>[2x]METIQELILSEENKTNIAVLNLGTNDRRNAVLILETALHLVEKYLGKII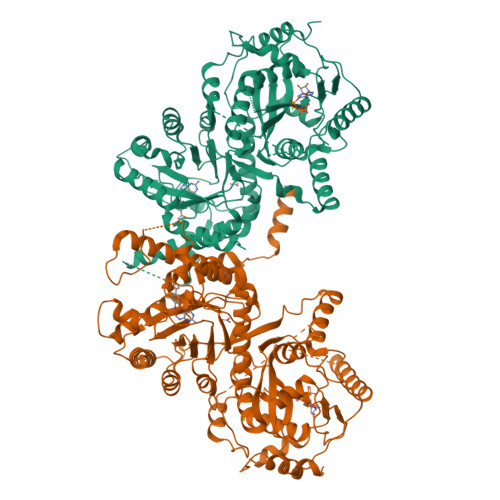NTSYLYETVPEYIVLDKKESCEKINKDCRIYDVNYINELMQNLEESKYEENKELIDKCEEYETFLKNGKVDNSILKEVNVENYLLECNNIIVKNDEIMKNNLSKYKDKYYTSYFYNLTVVVKTFVNDPLSMLVVIKYIEELMKRENVKEKEKFENRIIDIDILFFNDFTIFMKNIKLEKNMIYKILSKYIHLERDIKNGNDNMSKVNMDKDINLNNNNNIKKKNNNDIDCDCVDQKMNNHVNNKNYINSFRDPQEIINNMVDNIEFLSIPHVYTTHRYSILLCLNDMIPEYKHNVLNNTIRCLYNKYVSRMKEQYNINIKENNKRIYVLKDRISYLKEKTNIVGILNVNYDSFSDGGIFVEPKRAVQRMFEMINEGASVIDIGGESSGPFVIPNPKISERDLVVPVLQLFQKEWNDIKNKIVKCDAKPIISIDTINYNVFKECVDNDLVDILNDISACTNNPEIIKLLKKKNKFYSVVLMHKRGNPHTMDKLTNYDNLVYDIKNYLEQRLNFLVLNGIPRYRILFDIGLGFAKKHDQSIKLLQNIHVYDEYPLFIGYSRKRFIAHCMNDQNVVINTQQKLHDEQQNENKNIVDKSHNWMFQMNYMRKDKDQLLYQKNICGGLAIASYSYYKKVDLIRVHDVLETKSVLDVLTKIDQVKDPNSSSVDKLAAALEHHHHHH> GSPGIRLGSSEDNFAR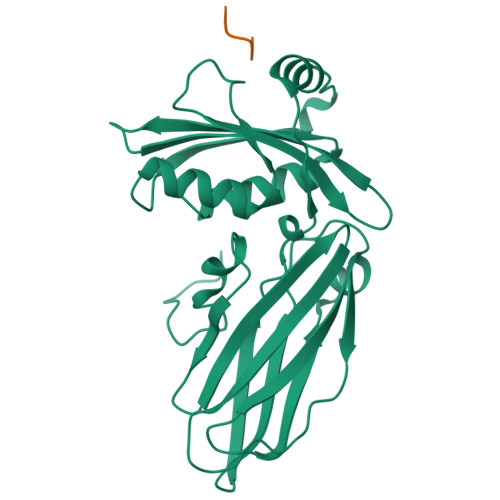FVCKNNGVLFENQLLQIGLKSEFRQNLGRMFIFYGNKTSTQFLNFTPTLICADDLQTNLNLQTKPVDPTVDGGAQVQQVVNIECISDFTEAPVLNIQFRYGGTFQNVSVKLPITLNKFFQPTEMASQDFFQRWKQLSNPQQEVQNIFKAKHPMDTEITKAKIIGFGSALLEEVDPNPANFVGAGIIHTKTTQIGCLLRLEPNLQAQMYRLTLRTSKDTVSQRLCELLSEQF;> GSDPFK>[2x]AEQVTKSVLFVCLG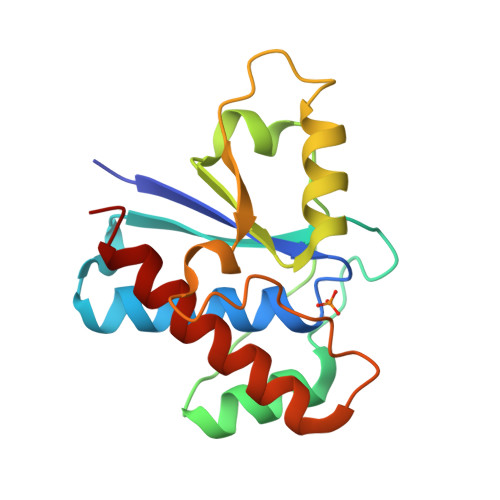NICRAPIAEAVFRKLVTDQNISDNWVIDSGAVSDWNVGRSPDPRAVSCLRNHGINTAHKARQVTKEDFVTFDYILCMDESNLRDLNRKSNQVKNCRAKIELLGSYDPQKQLIIEDPYYGNDADFETVYQQCVRCCRAFLEKVR>[4x]MAAGVAAWLPFARAAAIGWMPVANCPMPLAPADKNKRQDELIVLNVSGRRFQTWRTTLERYPDTLLGSTEKEFFFNEDTKEYFFDRDPEVFRCVLNFYRTGKLHYPRYECISAYDDELAFYGILPEIIGDCCYEEYKDRKRENAERLMDDNDSENNQESMPSLSFRQTMWRAFENPHTSTLALVFYYVTGFFIAVSVITNVVETVPCGTVPGSKELPCGERYSVAFFCLDTACVMIFTVEYLLRLFAAPSRYRFIRSVMSIIDVVAIMPYYIGLVMTNNEDVSGAFVTLRVFRVFRIFKFSRHSQGLRILGYTLKSCASELGFLLFSLTMAIIIFATVMFYAEKGSSAS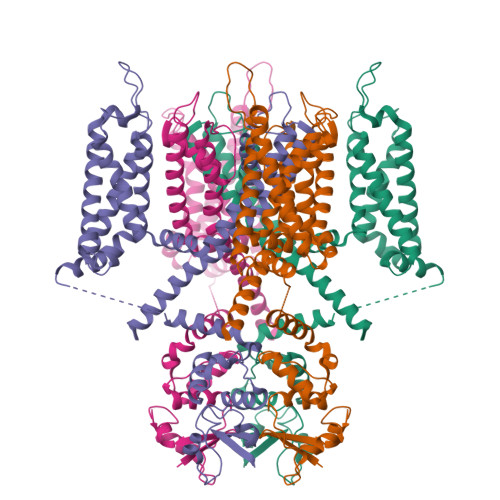KFTSIPASFWYTIVTMTTLGYGDMVPKTIAGKIFGSICSLSGVLVIALPVPVIVSNFSRIYHQNQRADKRRAQKKARLARIRVAKTGSSNAYLHSKRNGLLNEALELTGTPEEEHMGKTTSLIESQHHHLLHCLEKTTNHEFIDEQMFEQNCMESSMQNYPSTRSPSLSSHPGLTTTCCSRRSKKTTHLPNSNLPATRLRSMQELSTIHIQGSEQPSLTTSRSSLNLKADDGLRPNCKTSQITTAIISIPTPPALTPEGESRPPPASPGPNTNIPSIASNVVKVSALLEGGSSGGWSHPQFEK> MAGPEIVKLKKILREKAVPPGTEVPLDVMRKGMEKVAFKAADDIQVEQVTVAGCAAEWVRAPGCQAGKAILYLHGGGYVMGSINTHRSMVGEISRASQAAALLLDYRLAPEHPFPAAVEDGVAAYRWLLDQGFKPQHLSISGDSAGGGLVLAVLVSARDQGLPMPASAIPISPWADMTCTNDSFKTRAEADPMVAPGGINKMAARYLNGADAKHPYASPNFANLKGLPPLLIHVGRDEV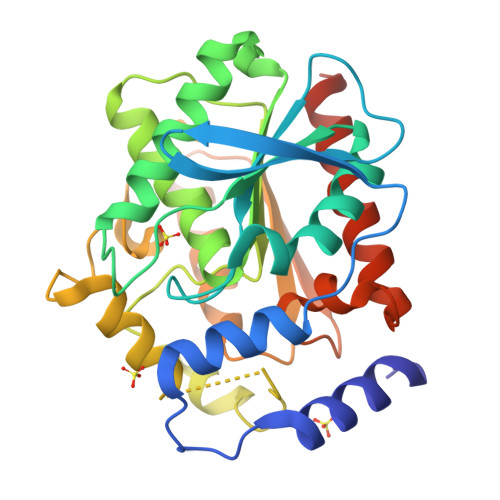LLDDSIKLDAKAKADGVKSTLEIWDDMIHVWHAFHPMLPEGKQAIVRVGEFMREQWAALAAALEHHHHHH> GLMSYKQFIQELEDDILPSEAERRYQEYKSEYITTQKRAFFNTH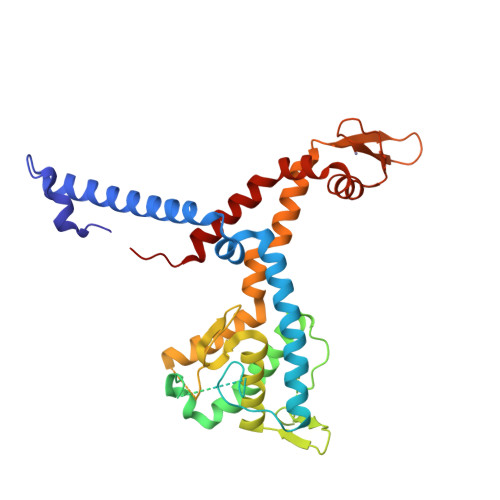KEEDWLKNKYHPTNLLSVIERRNDLAQKVAKDFLLDLQSGTLDLGPAVTALNKSGRTSEPNSEDEAAGVGKRKRHGMGGAKENELLSAAPKAPSFTSDPKRILTDVEQTQALVRKLDSEKKIEENVLQGSETEKSGREKLHSGSTGPVVIIRGLTSVKGLEGVELLDTLVTYLWRVHGLDYYGKVETNEAKGLRHVRAEGKVSDAKGDENESKFDSHWQERLKGQDPLEVMAAKEKIDAAATEALDPHVRKIRDEKYGWKYGCGAKGCTKLFHAAEFVYKHLKLKHTELVTELTTKVREELYFQNYLEHHHHHH> QEQFVKRRRDMLEHINLAMNESSLALEFVSLLLSSVKESTGMSSMSPFLRKVVKPSSLNSDKIPYVAPTKKEYIELDILNKGWKLQSLNESKDLLRASFNKLSSILQNEHDYWNKIMQSISNKDVIFKIRDRTSGQKLLAIKYGYEDSGSTYKHDRGIANIRNNIESQNLDLIPHSSSVFKGTDFVHSVKKFLRVRIFTKIESEDDYILSGESVMDRDSESEEAETKDIRKQIQLLKKIIFEKELMYQIKKECALLISYGVSIENENKVIIELPNEKFEIELLSLDDDSIVNHEQDLPKINDKRANLMLVMLRLLLVVIFKKTLRSRISSPHGLINLNVDDDILIIRPILGKVRFANYKLLLKKIIKDYVLDIVPGSSITETEVER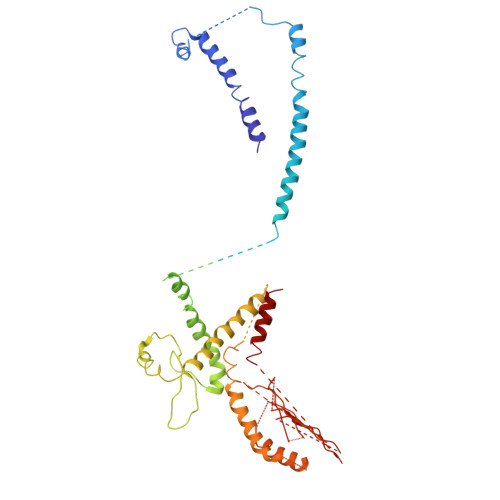EQPQENKNIDDENITKLNKEIRAFDKLLNIPRREXXXXXXXXXXXXXXXXXXXXXXXXXXXXXXXXXXXXXXXXXXXXXEVEDFLHFIVAEYIQQKKV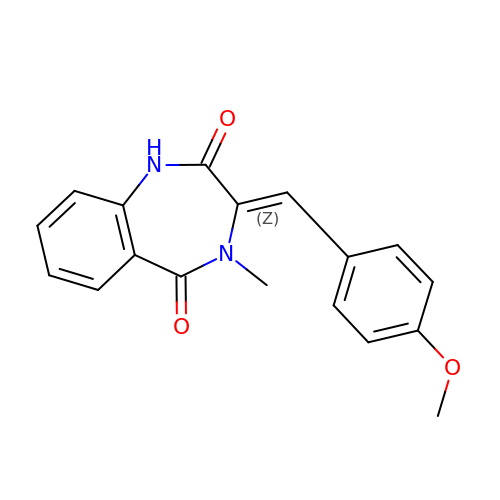4-Methoxydehydrocyclopeptin | C18 H16 N2 O3 | MWFWGXGLRBDFOQ-WJDWOHSUSA-N>[3x]MARGKQNSNQIQNNSNANGKRRKRNRRNRNPQTVPNFNPIVAKPTVAPLQTNIRSARSDVNAITVLNGSDFLTTVKVRGSNNLIDSKSRILVKQPISASSFLGTRISGLSQFWERYRWHKAAVRYVPAVPNTLACQLIGYIDTDPLDDPNVILDVDQLLRQATSQVGARQWNFSDTTTIPLIVRRDDQLYYTGQDKENVRFSQQGVFYLLQVTTLLNISGEAITNDLIS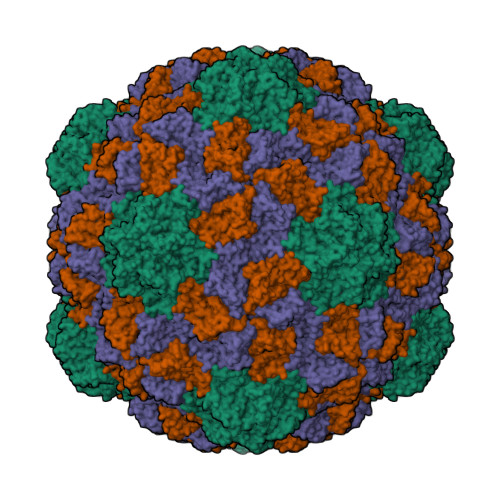GSLYLDWVCGFSMPQINPSPVEVSQLTYNADTIGNWVPPTELKQTYTQDITGLKPNSKFIIIPYMDRVSSEVLQKCTITCNEVDAVGSISYSDTSAIKCDGYILFQANSIGEATFTLVTDYQGAVDPKPYQYRIIRAIVGNN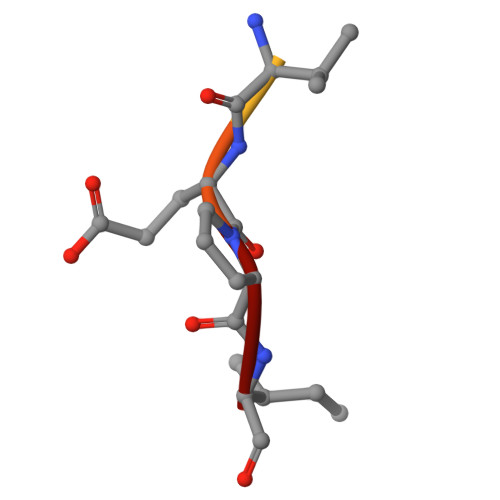> YPFVEPI N-[(2R)-1-(hydroxyamino)-3-methyl-3-(methylsulfonyl)-1-oxobutan-2-yl]-4-(6-hydroxyhexa-1,3-diyn-1-yl)benzamide 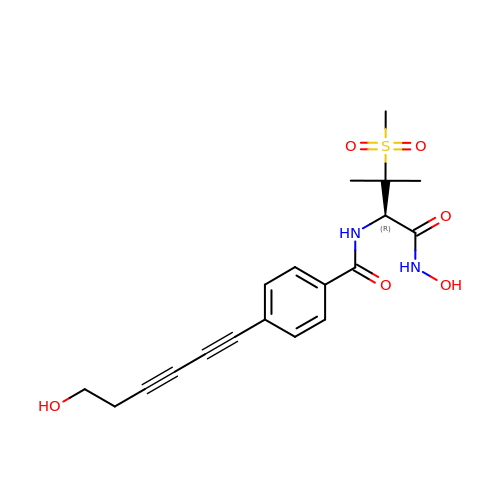| C19 H22 N2 O6 S | RFKFCSZMHYSIDP-MRXNPFEDSA-N> APPRLICDSRVLERYLLEAKEAEKITTGCAEHCSLNEKITVPDTKVNFYAWKRMEVGQQAVEVWQGLALLSEAVLRGQALLVKSSQPWEPLQLHVDKAVSGLRSLTTLLRALGAQKEA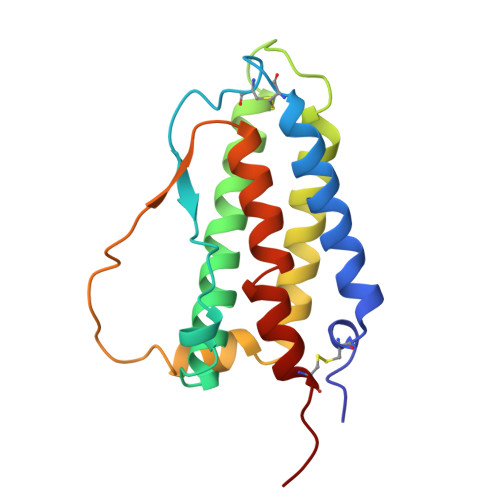ISNSDAASAAPLRTITADTFRKLFRVYSNFLRGKLKLYTGEACRTGDR> MDLRVGRKFRIGRKIGSGSFGDIYHGTNLISGEEVAIRLESIRSRHPQLDYESRVYKYLSGGVGIPFIRWFGREGEYNAMVIDLLGPSLEDLFNYCHRKFSFKTVIMLALQMICRVQYIHGRSFIHRDIKPDNFLMGVGRRGSTVHVIDFGLSKKYRDFNTHRHIPYRENKSLTGTARYASVNTHLGIEQSRRDDLESLGYMLIYFCKGSLPWQGLKATTKKQKY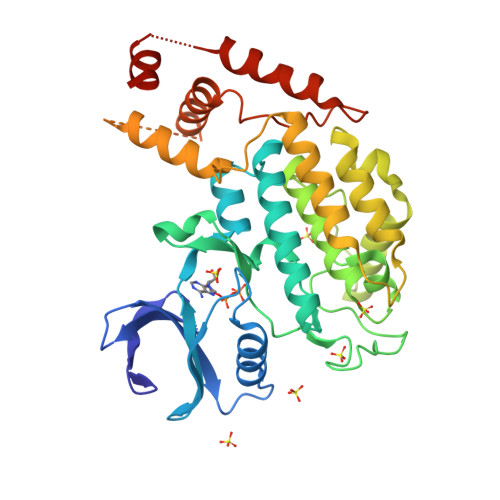DRILEKKLCISVETLCAGLPLEFSEYMNYCRNLKFDERPDYLYLARLFKDLSIKLEYHNDHLFDWTMLRYTKAMVEKQKDVLMLDTSSTANANKESGNNNNESNTTSNTKDSKNDSFNKVKLLAMKKFASHFHYCKNDDKHYPTPEEIKQQTVQNNNAAASLPPELLSAIDKGMENLK>[20x]MELFKDIKNLGKLVRLERIFNRESEKTVIVPMDHGVSNGPIKGLIDIRKTVNDVAEGGANAVLLHKGIVRHGHRGYGKDVGLIIHLSGGTAISPNPLKKVIVTTVEEAIRMGADAVSIHVNVGSDEDWEAYRDLGMIAETCEYWGMPLIAMMYPRGKHI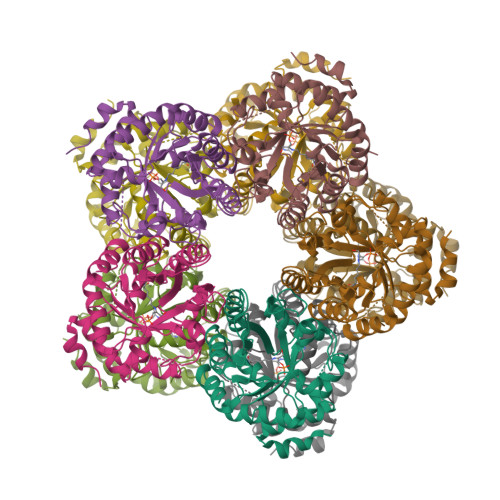QNERDPELVAHAARLGAELGADIVKTSYTGDIDSFRDVVKGCPAPVVVAGGPKTNTDEEFLQMIKDAMEAGAAGVAVGRNIFQHDDVVGITRAVCKIVHENADVEEALKEIRKK6-HYDROXYPROPYLTHYMINE | C8 H12 N2 O3 | 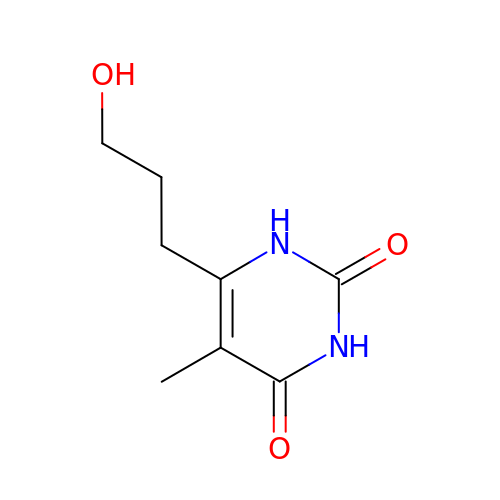OIEJBPVNLZZLGQ-UHFFFAOYSA-N> 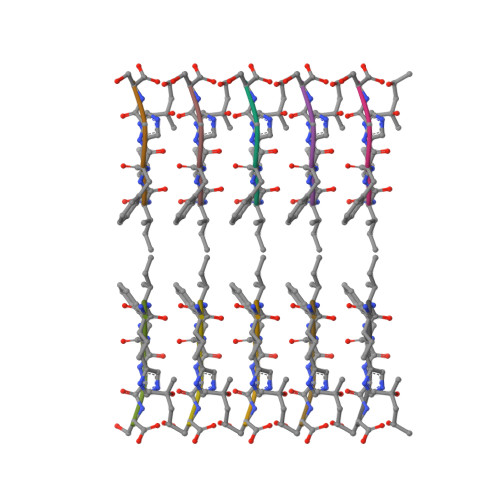IIHFGS> ARASPGSAASPRLREGPELSPDDPAGLLDLRQGMFAQLVAQNVLLIDGPLSWYSDPGLAGVSLTGGLSYKEDTKELVVAKAGVYYVFFQLELRRVVAGEGSGSVSLALHLQPLRSAAGAAAL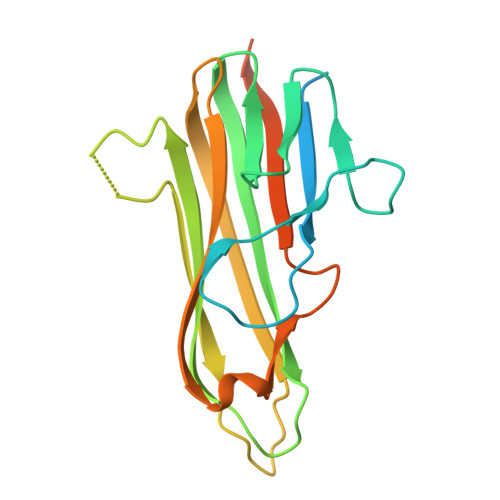ALTVDLPPASSEARNSAFGFQGRLLHLSAGQRLGVHLHTEARARHAWQLTQGATVLGLFRVTPEIPAGLPSPRSEGSHHHHHHHH The C-terminal, RNaseH-like catalytic domain contains a DDD/E motif, conserved in other transposases, recombination-activation gene (RAG) recombinases and retroviral integrases, which coordinates the metals required for catalysis. The eukaryotic mariner transposase Mos1 assembles as a homodimer and brings the Mos1 transposon ends together in a paired-end complex (PEC) for excision.

To establish the structural role of flanking DNA in accurate second strand cleavage, we have determined the crystal structure of a pre-TS cleavage Mos1 PEC. To trap the Mos1 PEC conformation before TS cleavage, we created a catalytically defective Mos1 transposase by mutating the second amino acid residue of the catalytic DDD triad (D249) to alanine. To prepare the pre-TS cleavage Mos1 PEC, we designed a DNA substrate incorporating the IR sequence plus five nucleotides of unpaired TS-flanking DNA, including the TpA dinucleotide abutting the transposon end. Crystals of the pre-TS cleavage Mos1 PEC diffracted X-rays to 3.09 Å resolution and exhibited C-centred orthorhombic symmetry. The pre-TS cleavage Mos1 PEC structure contains a transposase dimer and two DNA substrates arranged in trans. Each TS is routed through an active site and the backbone is intact at the IR-flanking DNA junction, consistent with a pre-TS cleavage state. As predicted, we do not observe Mg2+ ions bound to either site 1 or site 2 in the active site of the catalytically defective T216A/D294A mutant transposase. The TS backbone twists as it passes through the active site; T57 is de-stacked from adjacent nucleotides with the base flipped into a hydrophobic pocket lined by residues of the conserved WVPHEL and YSPDL motifs. The aromatic rings of H122 and Y276 stack at the base of the pocket, so that only a pyrimidine base is accommodated, while a hydrogen bond between the backbone carbonyl of P121 and the N3H of T57 confers base specificity. By contrast, there are no base-specific interactions with A58, providing a molecular explanation for the report that TS cleavage tolerates any base in this position.

>[3x]FVPNKEQTRTVLIFCFHLKKTAAESHRMLVEAFGEQVPTVKTCERWFQRFKSGDFDVDDKEHGKPPKRYEDAELQALLDEDDAQTQKQLAEQLEVSQQAVSNRLREMGKIQKVGRWVPHELNERQMERRKNTCEILLSRYKRKSFLHRIVTGDEKWIFFVNPKRKKSYVDPGQPATSTARPNRFGKKTMLCVWWDQSGVIYYELLKPGETVNAARYQQQLINLNRALQRKRPEYQKRQHRVIFLHANAPSHTARAVRDTLETLNWEVLPHAAYSPDLAPSDYHLFASMGHALAEQRFDSYESVKKWLDEWFAAKDDEFYWRGIHKLPERWEKCVASDGKYFE>SQNLTCNSNDLKALEGFMRGLESSIDGWKWNESSSFSSNCCDWVGISCKSSVSLGLDDVNESGRVVELELGRRKLSGKLSESVAKLDQLKVLNLTHNSLSGSIAASLLNLSNLEVLDLSSNDFSGLFPSLINLPSLRVLNVYENSFHGLIPASLCNNLPRIREIDLAMNYFDGSIPVGIGNCSSVEYLGLASNNLSGSIPQELFQLSNLSVLALQNNRLSGALSSKLGKLSNLGRLDISSNKFSGKIPDVFLELNKLWYFSAQSNLFNGEMPRSLSNSRSISLLSLRNNTLSGQIYLNCSAMTNLTSLDLASNSFSGSIPSNLPNCLRLKTINFAKIKFIAQIPESFKNFQSLTSLSFSNSSIQNISSALEILQHCQNLKTLVLTLNFQKEELPSVPSLQFKNLKVLIIASCQLRGTVPQWLSNSPSLQLLDLSWNQLSGTIPPWLGSLNSLFYLDLSNNTFIGEIPHSLTSLQSLVSKENAVEEPSPDFPFFKKKNTNAGGLQYNQPSSFPPMIDLSYNSLNGSIWPEFGDLRQLHVLNLKNNNLSGNIPANLSGMTSLEVLDLSHNNLSGNIPPSLVKLSFLSTFSVAYNKLSGPIPTGVQFQTFPNSSFEGNQGLCGEHASPCHITDQSPHGSHHHHHH[2x];>MGRKKFEAFGFVCLISLLLLFNSLWLASSNMEGDALH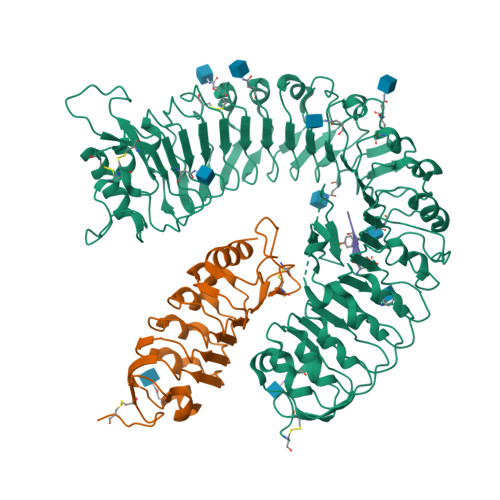SLRANLVDPNNVLQSWDPTLVNPCTWFHVTCNNENSVIRVDLGNADLSGQLVPQLGQLKNLQYLELYSNNITGPVPSDLGNLTNLVSLDLYLNSFTGPIPDSLGKLFKLRFLRLNNNSLTGPIPMSLTNIMTLQVLDLSNNRLSGSVPDNGSFSLFTPISFANNLDLCGPVTSRPCPGSHHHHHH[2x];>YIYTQ[2x]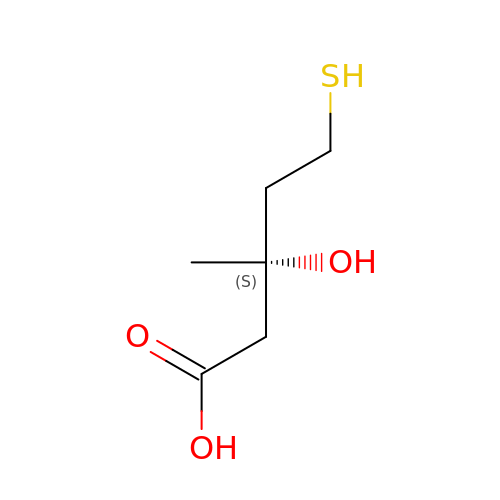(3S)-3-hydroxy-3-methyl-5-sulfanylpentanoic acid | C6 H12 O3 S | MCHPXVGJHBKMNR-ZCFIWIBFSA-N>[6x]MTEDRLSAEDKKFLEVERALKEAALNPLRHATEELFGDFLKMENITEICYNGNKVVWVLKNNGEWQPFDVRDRKAFSLSRLMHFARCCASFKKKTIDNYENPILSSNLANGERVQIVLSPVTVNDETISISIRIPSKTTYPHSFFEEQGFYNLLDNKEQAISAIKDGIAIGKNV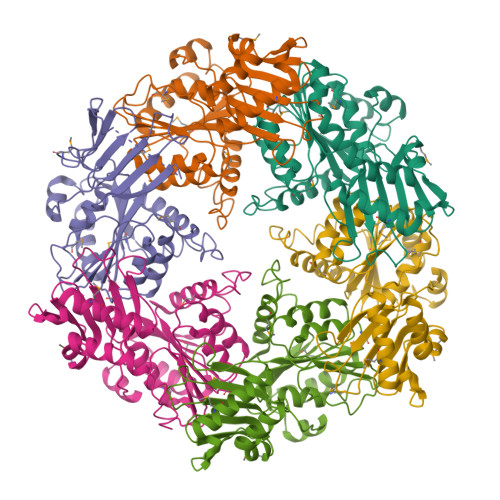IVCGGTGSGKTTYIKSIMEFIPKEERIISIEDTEEIVFKHHKNYTQLFFGGNITSADCLKSCLRMRPDRIILGELRSSEAYDFYNVLCSGHKGTLTTLHAGSSEEAFIRLANMSSSNSAARNIKFESLIEGFKDLIDMIVHINHHKQCDEFYIKHR>MAHHHHHHMAKIVVTGGAALHGEVSISGAKNAVLPILCATLLADEPVEITNVPHLHDVVTTVKLLGELGAKVTIDQGTLSRGSAIVVDPRPVNQHVAPYELVKTMRASILVLGPLLARFGAAEVSLPGGCAIGSRPVDQHIKGLQALGAEIVVENGFIKASAKRLKGGHFTFDMVSVTGTENVLMGAVLAEGTTVLDNCAMEPEVTDLAHCLIALGAKIEGLGTARLVIEGVERLSGGRHEVLPDRIETGTFLVAAAMTGGKVTVNRARPNTMDAVLSKLVEAGAKIETTDDSITLDMQGRRPKAVNLTTAPYPAFPTDMQAQFMALNCVADG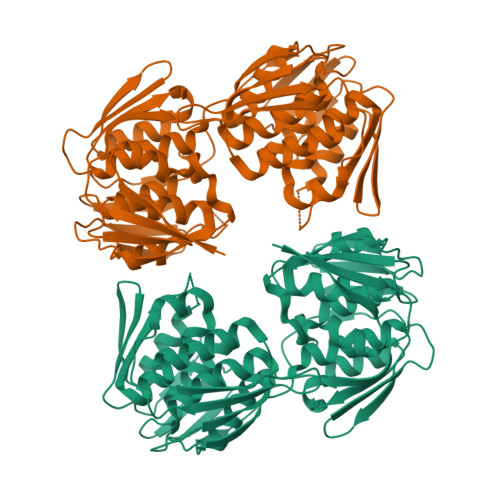VGVINETIFENRFMHVNELLRLGADIQVEGHTAIVRGSEHLSGAPVMATDLRASASLILAGLMASGDTTIDRIYHLDRGYENIEEKLSSLGATIRRVP[2x]>[2x]SETQECLFFNANWERDRTNQTGVEPCYGDK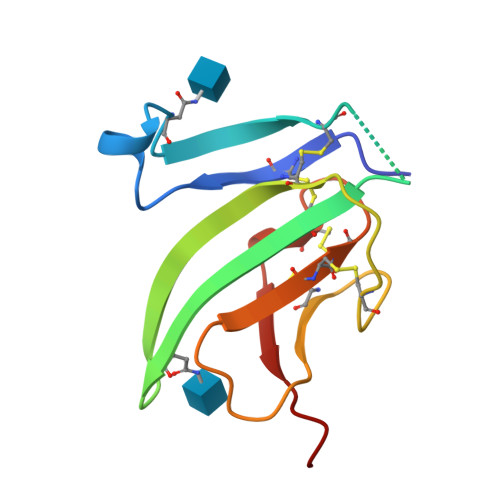DKRRHCFATWKNISGSIEIVKQGCWLDDINCYDRTDCIEKKDSPEVYFCCCEGNMCNEKFSYFPEME>SAGSLAADEQLDGPVLAMLTTAQQQQGSGDLNSAAASLERAQRIAPREPQVLYRLAQVRLAQGDAAQAEQVARRGLSYANGRPALQAGLWELIAQAREKQGDSAGAA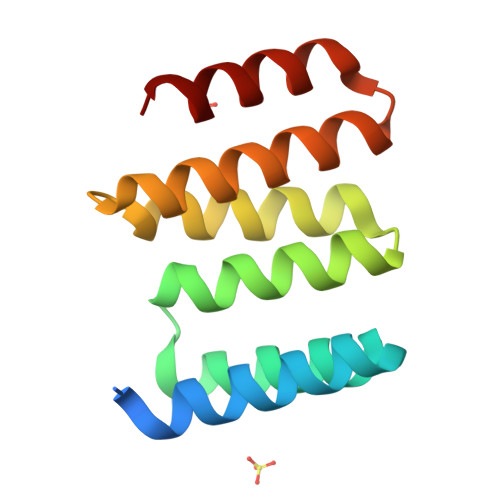LARQKAKVS[8x]>[6x]GSHMDSLIAQCSPEADTLLTDNPSKANRILEDPDYSLVKALQMAQQNFVITDASLPDN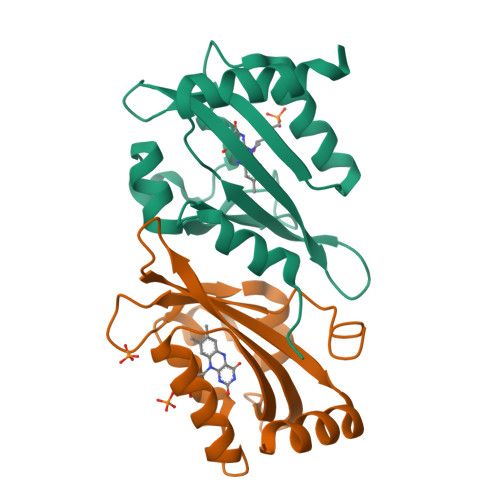PIVYASRGFLTLTGYSLDQILGRNCRFLQGPETDPRAVDKIRNAITKGVDTSVCLLNYRQDGTTFWNLFFVAGLRDSKGNIVNYVGVQSKVSEDYAKLLVNEQNIEYK>[2x]IFPKQYPIINFTTAGATVQSYTNFIRAVRGRLTTGADVRHEIPVLPNRVGLPIN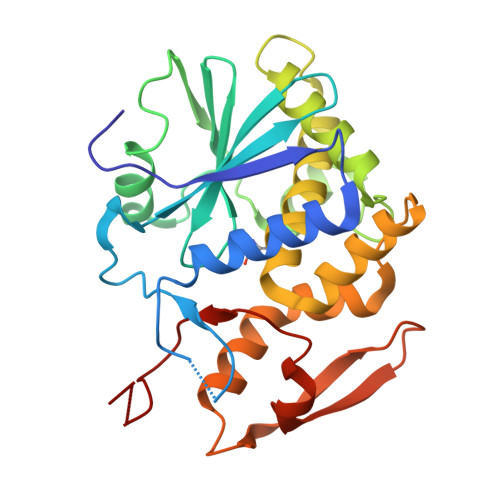QRFILVELSNHAELSVTLALDVTNAYVVGYRAGNSAYFFHPDNQEDAEAITHLFTDVQNRYTFAFGGNYDRLEQLAGNLRENIELGNGPLEEAISALYYYSTGGTQLPTLARSFIICIQMISEAARFQYIEGEMRTRIRYNRRSAPDPSVITLENSWGRLSTAIQESNQGAFASPIQLQRRNGSKFSVYDVSILIPIIALMVYRCAPPPSSQF> GGKKKNYQRYPKPPYSYLAMIAMVIQNSPEKKLTLSEILKEISTLFPFFKGNYKGWRDSVRHNLSSYDCF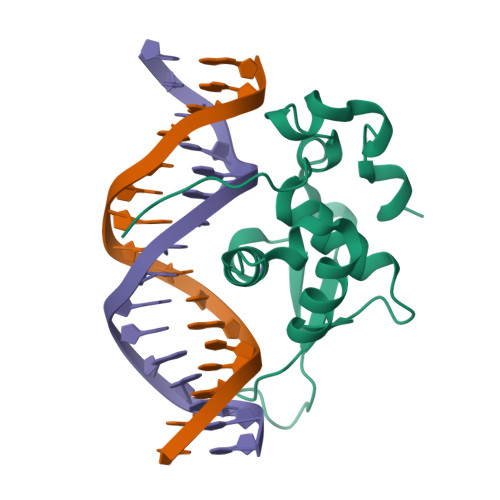VKVLKDPGKPQGKGNFWTVEVNRIPLELLKRQNTAVSRQDETIFAQDLAPYIFQG UNDECANAL | C11 H22 O | 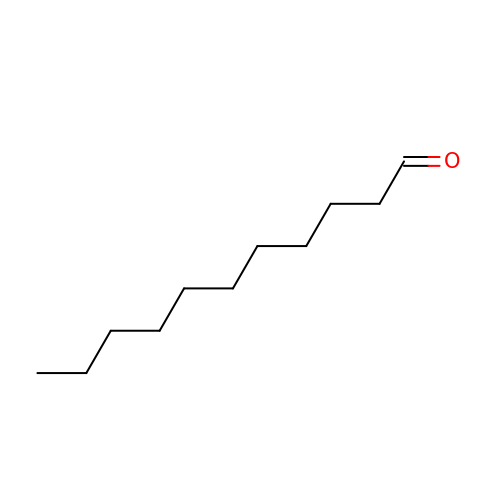KMPQYAYAQWNLME-UHFFFAOYSA-N>[2x]MQLREIRNCLLKCISECSERGLVYAVRWAAEMLNGMNPIEMEHIPFSSTPTGEFDLDPDMANEKLLEVEEKNIYLLAKSYFDCKEFERAAYTLQNCKSSKSIFLRLYSKYLAGEKKSEEENETLLNTNLTLSSTNREFYYISEVLESLHYQGNKDPYLLYLSGVVYRKRKQDSKAIDF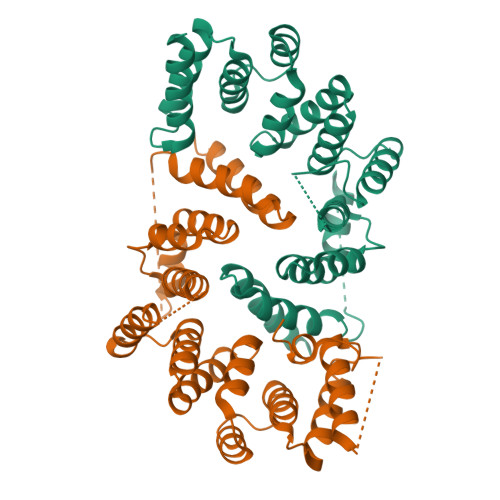LKSCVLKAPFFWSAWLELSLSIDSLETLTTVVSQLPSTHIMTKIFYVYASHELHQVNSSAYEKLAEAEIIFPNSRYLKTQRALLTYDSRLFDEAESLFENILTNDPAENLYFQ>MSTAAEGGAIRRAGHEPRYDLAQLPPAPPTTVAVIEGMATGAPQRVVAQADAAARVSELFVDPQQRERISRIYDKTRIDTRRMAVDPLDDEFDEFRREPATIRDRMNLFYQHAVPLAVDVAARALDGLPYAPDEIGQLVFVTSTGFIAPGVDVEIVKQLGLPRSISRVVVNFMGCAAAMNAIRTATNYVRAHPSMKALVVCIELSSVNAVFADDINDVVIHSLFGDGCGALVIGASQVQQPLPAGNVVIRSSFSQLLDDSEDGIVLGVNHDGITCELSENLPSYIYRSVDPVVAEM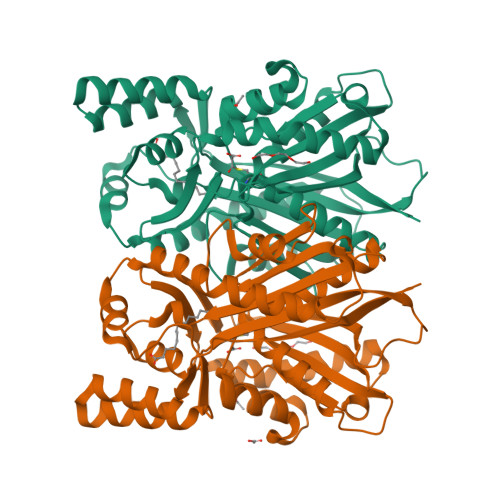LRDNGLSKADIDLWAIHPGGPKIIEQSARSLGIPVGRAVQSWDVLAQFGNMLSVSLIFVLEMMVAQAESDKPISTGVAFAFAPGVTVEGMLFDIIRRGNSSSVDKLAAALEHHHHHH[2x]(2R,3S,4R,5R)-2-(hydroxymethyl)-5-[6-(4-phenylpiperazin-1-yl)-9H-purin-9-yl]tetrahydrofuran-3,4-diol | C20 H24 N6 O4 | 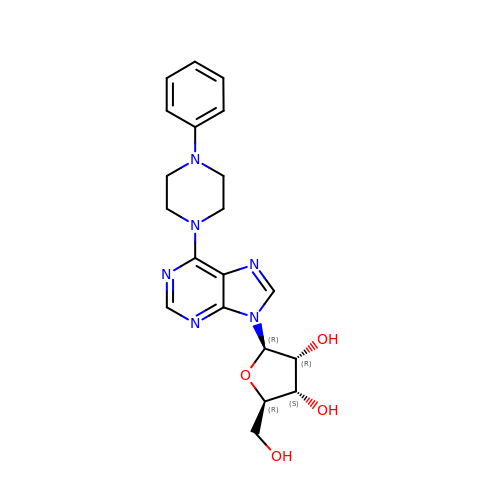FVRJZHPJEJJPPT-WVSUBDOOSA-N> QLATKAAR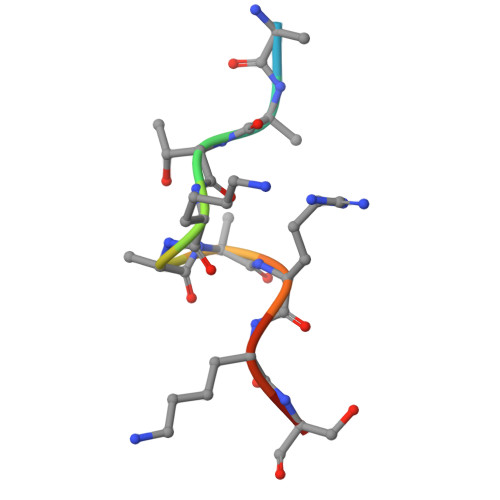KSA N-hydroxycyclohexanecarboxamide | C7 H13 N O2 | 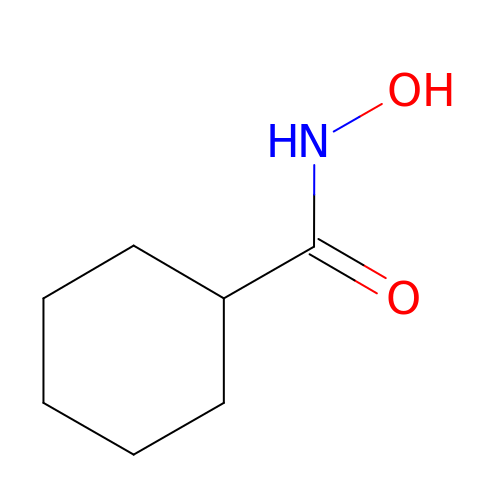RFWDAWXPYZTVSN-UHFFFAOYSA-N>[2x]FNCTSSSATVHWLGDKPTYHAGVTFGLPWPQGKYRPQETSFSLTGDTEDKSELQSWATGYWADGSLKWTAHAIAESNQIYDQYTVTASSLGCVKSSSSSSESSAPNSSIVVTDNSDALTVNTGEV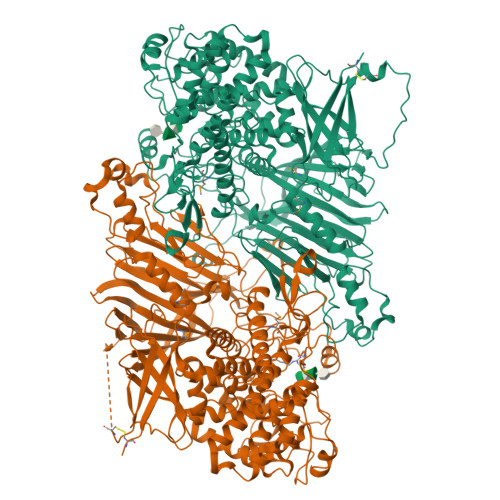AVSFPKGGNVIIGDIKTKSGKVIGANGRLVLQSQDSVPDNFDNRANSPIQYSNFDGNINEVFVNQTSARTLVTVRGNHTVTDGTDHDPWLPFVVRFYLYANSATIKVMHSIVFDGDENDFITGLGIRFDVPLKGEEYYDRHIRFAGVDGGIFNEAVQGITGLRRDPGEEIRAAQFAGQKLADTETWEPRVSTRLKWIPTWADYGLTQLTADGFGLKKRTKAGQSWVNIPSGTRAEGLAYLGGATQGGLAVGLRDFWKRYPVGLDISNAASDTGELTLWLYSPAAEPLDLRPFHDGLGQDGYEDQLDALEITFEDWEPGFDTPYGIARTSEVYLFAFDQTPTSDKLASLTAYMNDPPVLVAEPKYIHETQALGEYWALPGSASPAAATLEDRLQFIFDFYKGQIEQRRWYGFLDYGDFMHTYDPDRHTWRYDVGGYAWDNSELSPDLFFWLYFLRTGSKDAYRFAEALTRHTGEVDVYHIGDWKGLGTRHGVQHWSDSAKQARISQPQYRKYFFYLSGGDERVGELLEELLDTDKTYGELDPQRKVRTDGWEPSPNSTVSFGLGTDWSGLAAGWLIEWERRGPRWEEAKTKLTNTIAGIANLTNGFVTGSGLYDPVTWTLGPPPSDPGNRGNVSISHLNAVFGLPEVVSEAIAYLADDIPKGFKQAWLDYCYYYHASASEQKDRYGVSFSKISLLQAHSRLAAYAAYETKNKTLALRAWKDFYASDGLLPDAPWNITHVDGSDVLVPVDEAAWLATNDIAQYGLAVIQNLAYVSDSLDDYQS> MGQNHHEVVKFMDVYQRSYCHPIETLVDIFQEYPDEIEYIFKPSCVPLMRCGGCCNDEGLECVPTEESNITMQIMRIKPHQGQHIGEMSFLQHNKCECRPKK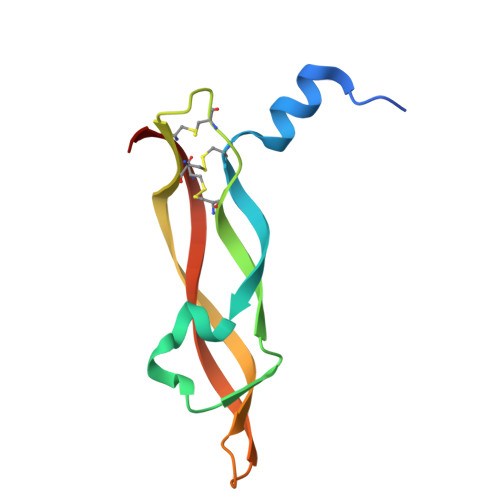D> MASDVYLIFSTCPDLPSAEIISRVLVQERLAACVTQLPGAVSTYRWQGKIETTQEIQLLIKTNAVHVNAAITRLCALHPYRLPEAIAVQVSVGLPEYLTWI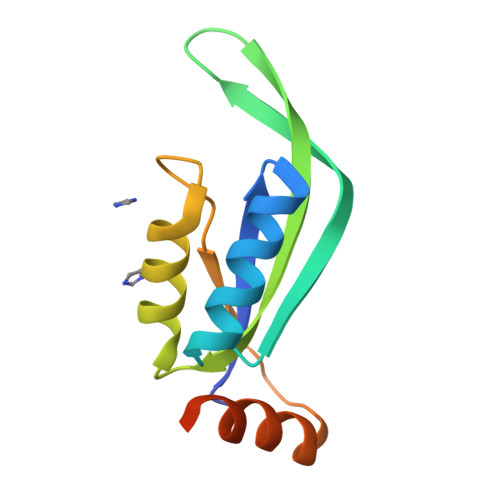NTEIDEEYSLPHHHHHH> LPDSVDWREKGCVTEVKYQGSCGACWAFSAVGALEAQLKLKTGKLVTLSAQNLVDCSTEKYGNKGCNGGFMTTAFQYIIDNKGIDSDASYPYKAMDQKCQYDSKYRA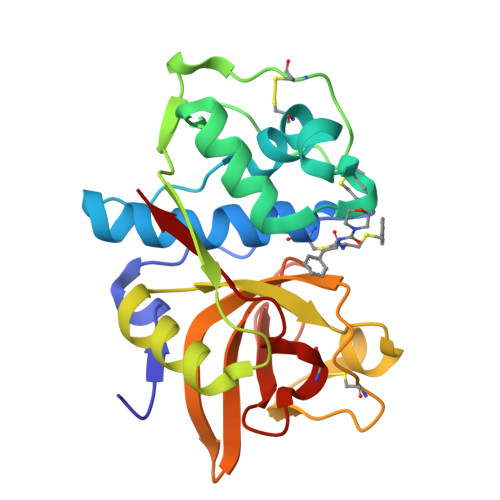ATCSKYTELPYGREDVLKEAVANKGPVSVGVDARHPSFFLYRSGVYYEPSCTQNVNHGVLVVGYGDLNGKEYWLVKNSWGHNFGEEGYIRMARNKGNHCGIASFPSYPEI GUANINE 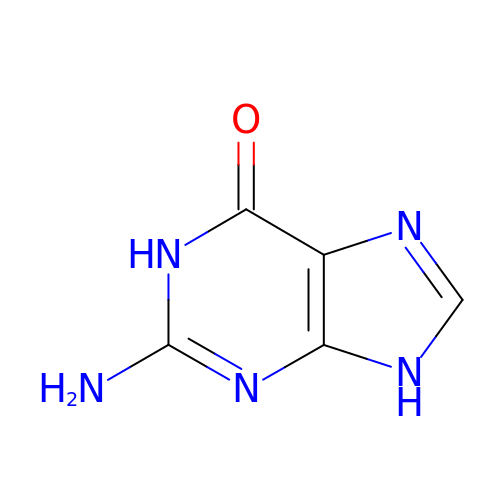| C5 H5 N5 O | UYTPUPDQBNUYGX-UHFFFAOYSA-N>SNAMNDIVASTQLPNTIKTITNDLRKLGLKKGMTVIVHSSLSSIGWISGGAVAVVEALMEVITEEGTIIMPTQSSDLSDPKHWSRPPVPEEWWQIIRDNVPAFEPHITPTRAMGKVVE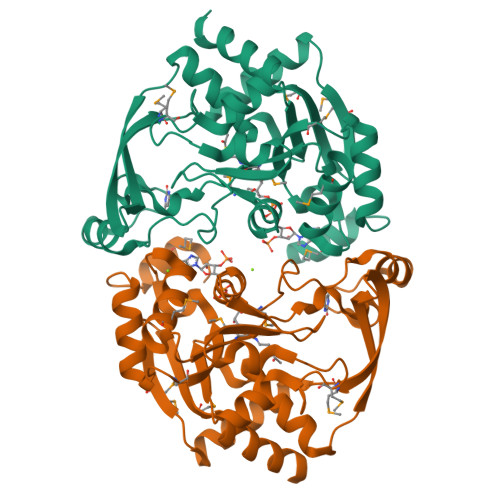CFRTYPNVVRSNHPLGSFAAWGRHAEEITVNQSLSMSLGEESPLRKIYDLDGYILLIGVGYDSNTSVGLSEVRSGACELIKVGAPIIENGERVWKEFVDMDYDSDKFVEIGVEFEQKGTVTMGKIGNAKCRLMKQRDIVDFGTEWFRKKN[4x]> DDKMDYDFKVKLSSERERVEDLFEYEGCKVGRGTYGHVYKAKRKDGKDDKDYALKQIEGTGISMSACREIALLRELKHPNVISLQKVFLSHADRKVWLLFDYAEHDLWHIIKFHRASKANKKPVQLPRGMVKSLLYQILDGIHYLHANWVLHRDLKPANILVMGEGPERGRVKIADMGFARLFN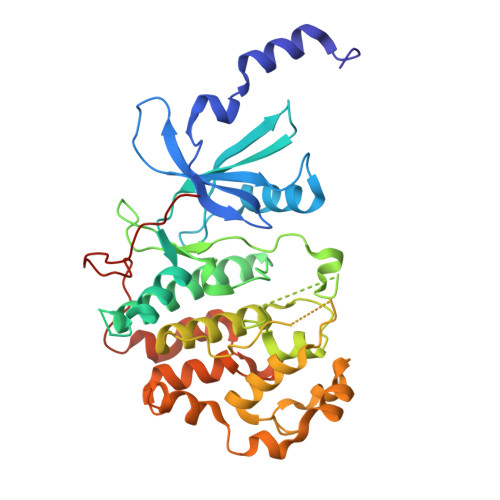SPLKPLADLDPVVVTFWYRAPELLLGARHYTKAIDIWAIGCIFAELLTSEPIFHCRQEDIKTSNPYHHDQLDRIFNVMGFPADKDWEDIKKMPEHSTLMKDFRRNTYTNCSLIKYMEKHKVKPDSKAFHLLQKLLTMDPIKRITSEQAMQDPYFLEDPLPTSDVFAGCQIPYPKREFLTEEPPLKK>MTHEEHHAARTLGVGKAIAVLTSGGDAQGMNAAVRAVVRVGIFTGARVFFVHEGYQGLVDGGDHIREATWESVSMMLQLGGTVIGSARCKDFREREGRLRAAHNLVKRGITNLCVIGGDGSLTGADTFRSEWSDLLSDLQKAGKITAEEATRSSYLNIVGLVGSIDNDFCGTDMTIGTDSALHRITEIVDAITTTAQSHQRTFVLEVMGRHCGYLALVTSLSCGADWVFIPECPPDDNWEDHLCRRLSETRTRGSRLNIIIVAEGAIDRNGKPITSEGVKDLVVRRLGYDTRVTVLGHVQRGGTPSAFDRILGSRMGVEAVMALLEGTPDTPACVVSLSGNQAVRLPLMECVQVTKDVTKAMDEKRFDEAMKLRGRSFMNNWEVYKLLAHIRPPAPKSGSYTVAVMNVGAPAAGMNAAVRSTVRIGLIQGNRVLVVHDGFEGPAKGQIEEAGWSYVGGWTGQGGSKLGSKRTLPKKSFEQISANITKFNIQGLVIIGGFEAYTGGLELMEGRKQFDELCIPFVVIPATVSNNVPGSDFSVGADTALNTICTTCDRIKQSAAGTKRRVFIIETMGGYCGYLATMAGLAAGADAAYIFEEPFTIRDLQANVEHLVQKMKTTVKRGLVLRNEKCNENYTTDFIFNLYSEEGKGIFDSRKNVLGHMQQGGSPTPFDRNFATKMGAKAMNWMAGKIKESYRNGRIFANTPDSGCVLGMRKRALVFQPVTEL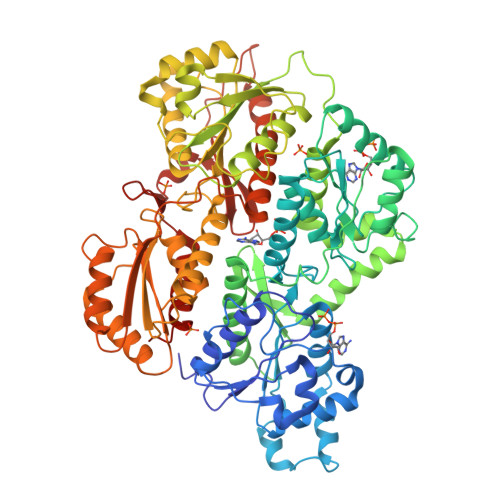QNQTDFEHRIPKEQWWLKLRPILKILAKYEIDLDTS[2x]> CDLPQTHNLRNKRALTL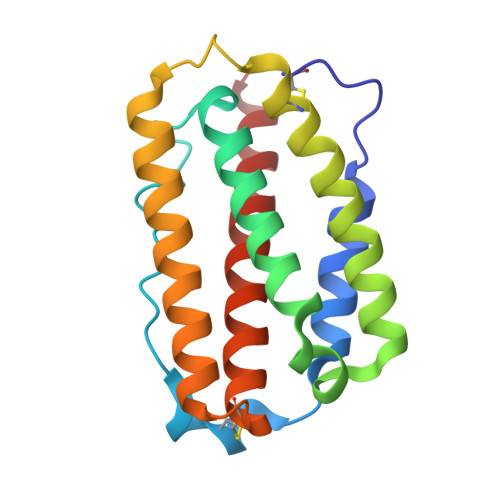LVKMRRLSPLSCLKDRKDFGFPQEKVGAQQIQEAQAIPVLSELTQQVLNIFTSKDSSAAWNATLLDSFCNEVHQQLNDLKACVMQQVGVQESPLTQEDSLLAVRKYFHRITVYLREKKHSPCAWEVVRAEVWRALSSSVNLLARLSKEE>[4x]QTLDIQRGATLFNRACIGCHDT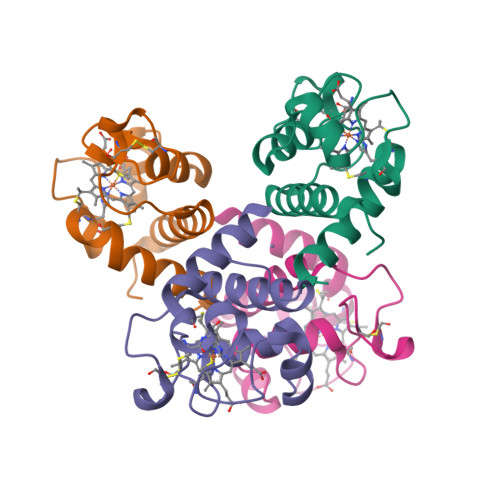GGNIIQPGATLFTKDLERNGVDTEEEIYRVTYFGKGRMPGFGEKCTPRGQCTFGPRLQDEEIKLLAEFVKFQADQGWPTVSTD The E.coli Fic protein EcFicT forms a tight complex with its cognate antitoxin EcFicA. EcFicT adopts the conserved Fic fold, but with a distinct active site signature motif and an additional hydrophobic binding pocket in the vicinity of the active site loop. EcFicA forms two parallel α-helices that tightly embrace EcFicT. According to this classification, EcFicT belongs to class I with the inhibitory helix provided by EcFicA, a small protein coded immediately upstream of the ecficT gene.

For EcFicT in complex with the antitoxin mutant EcFicAE28G, crystals of the monoclinic space group C2 were obtained that diffracted to 2.4 Å, containing three toxin-antitoxin complexes per asymmetric unit. Strikingly, mutation of the putative inhibitory glutamate residue E28 (EcFicAE28G) decreases the melting temperature of the complex by 10°C compared to the wild-type complex. The peaks of the first derivative of the melting curve of EcFicTAE28G and EcFicTG55RAE28G appear to broaden towards lower temperature, indicating that the E28G mutation may weaken the complex stability, resulting in a partial dissociation of EcFicAE28G from EcFicT. EcFicTAE28G crystallized in the space group C2 with three complexes per asymmetric unit. The structure of this mutant is virtually identical to that of EcFicTG55RA, except for disorder of residues 83–86 at the tip of the flap. Despite distinct crystal packings, the structures of EcFicTG55RA and EcFicTAE28G are virtually identical (root mean square deviation (rmsd) of 0.59 Å for 232 Cα-atoms). In particular, the interactions formed between the Fic protein and the antitoxin are the same, giving confidence that they are physiological and also occur in solution. The Ramachandran angles of R55 (Φ, Ψ = -120.7, -160.4) are virtually the same as those of the G55 wild-type residue (Φ, Ψ = -133.6, -155.8 as measured in the EcFicTAE28G structure). Though the side-chain truncation in EcFicAE28G increases the size of the putative substrate binding site, it may not be sufficient to allow productive substrate binding and relieve the inhibition of EcFicT. Because of the hydrophobic pocket on the left-hand side of the active site that may accommodate a different substrate, de-binding of EcFicA or more drastic mutations may be required to allow ligand binding.

>[3x]MGSSHHHHHHSQDPNSSSARLQVEMGDKFGEGRDPYLYPGLDIMRNRLNIHQQQRLEQAAYEMTALRAATIELGPLVRGLPHLRTIHRQLYQDIFDWAGQLREVDIYQGDTPFCHFAYIEKEGNALMQDLEEEGYLVGLEKAKFVERLAHYYCEINVLHPFRVGSGLAQRIFFEQLAIHAGYQLSWQGIEKEAWNQANQSGAMGDLTALQMIFSKVVSEAGESE;>MAYPYDVPDYAAAVKKLTDKQKSRLWELQRNRNFQASRRLGGVEMPLVTLTAAEALARLEELRSHYER[3x]>[2x]MALILTFLGKSGVARTKIAIAAAKLLASQGKRVLLAGLAEPVLPLLLEQTLTPDPQQIAPNLEVVQFQSSVLLERNWEEVKKLEAQYLRTPIIKEVYGQELVVLPGMDSALALNAIREYDASGKYDTIVYDGTGDAFTLRMLG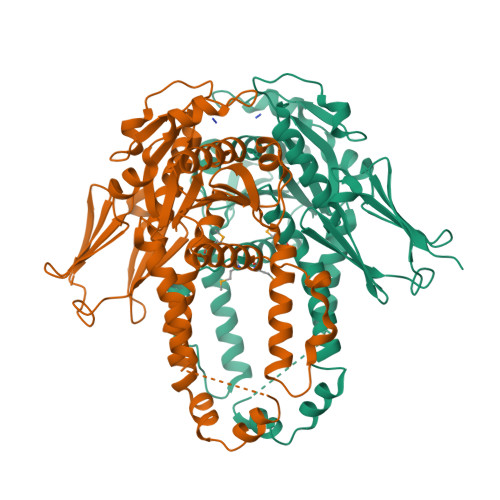LPESLSWYVRRFRQLFVNSDLGKTIAESPLIQPLISSFFNVNWTADNFAQPTNQVNNFLDKGKEALADPKRVAAFLVTTADPLEVVSVRYLWGSAQQIGLTIGGVIQVSSQTEGDLSAEFTPLSVTVVPDVTKGDWQPLIDALPNFVEQAEQAPKPITIDTHNRQVRLFLPGFDKKQVKLTQYGPEVTVEAGDQRRNIFLPPALSGRPITGAKFQNNYLIISFLEHHHHHH>XFAAAVGLVAPQVPAP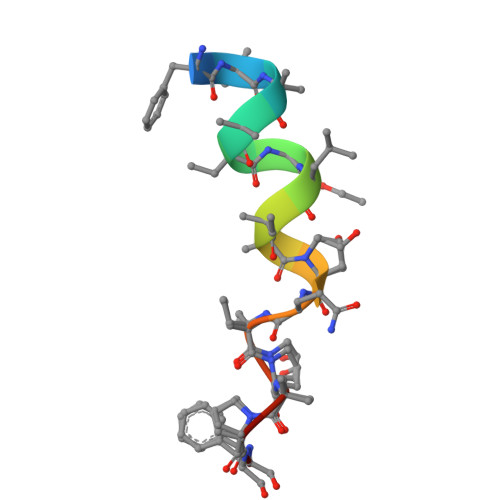F[2x]>[4x]GSGSMNRTVNATTPLGDKLKFKSLKGHEQLSDLFEWTVEFVSDSPGLVLEDLLGKTISLEVETSAAPRYMHGVITAFKLVHRETQTRRYYIYEATVRPWLWYSTQVTDNRIFQDQTAVQIITQVLQAYDYPIENRLVGQYRKWGYSVQFQESDFNFISRLMEHEGIYYWFRHEKDQHVLVLMDDAHSHAPLPVMPDIPFYPDDTRSVPLEEYIRDWQIAGELTPTTYSTMDYDFQKPQAEMSARRWVKNQNTQGLDLDWYDPMGGYVDSADSDHYARVHLESMQCLQEQAWAVSNVRNLAPGYTFSLKYYPNSEENKSYLILRAEYDFRDPSYASAGGVQENATFVIRSQHIPASVQFRAPRSTPAPRMSGPQTATVVGPDGQEIWTDKYGRIKVQFHWDRQGAMDENSSCWLRVSSPWAGGGFGGVQIPRVREEVVVDFINGDVDRPIAVGRVYNASNMPPVSLPENATQSGFLTRTKNGTPENANKMLFEDSQGNELLSMVAEKDMNTHVKNNQQHDVVGNAVSSIGGLRSHTAHSTSSITMASGAVKSYQSNHNRTVQASLDDSVGGNLEQTLSDGVDETITGAHSHTVSGAASHQLLGLHVNTTTQDVETVNGTVTETVSADETTNVT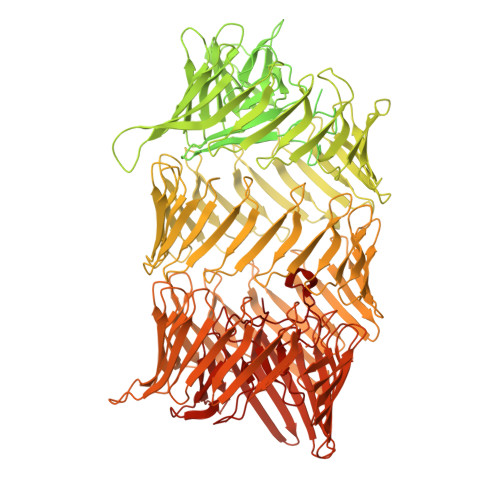SSSELEAADITLETPSLYKESTKQDININAGGSLDIQSTGPGIIQTPTDIEKESPANLEAAVMLDNNTVNREDKYILKLNLDAMSDVMVSGAKTDRNIADLAFYGMGGTMQLANVGIYGASIQMGSSDQKMGLASLSITGLELDKGFKIKTMGAGGRSGYKGKHRAAGGGRGPRGGKGGRHRAGNKGDPKKPHADCKECRGRVGGSIGLDVGDERFSHLDFVLPGVFPLEWNRTYRSNMTAKDGQGELGPRWITAFTLVVLPLETGGYEYISEVGRAVSVIELEPGQEWYDRTEELIWRRPDVDTLEVSQKYQRTETFERSGDVFRLKTIADRAGNQAQLIYDAENGFLVRVETAIQTVHLDHDAHGRITTIWHEVTGDDGTPLRRTLARYQYDEAHDLVAAVDQYERTHTYAYQNHLITRYSDKTGRGINLEWDGDHPQAKCVREYRDDGSNLLRFRWDESESKTYVTDALSATTVYTFDAHNYIIHIDFADGTRQSRIRDEFHNIVEVRYPDDSFEKYEYDEFDNILKLTRADHTTVGWEYDQYSQITKIVDPGGNIWTRDYDQFGNMIRETDPKGHTSEFQYTAEGLLIQSVNPAGGVSTLSYNPAGLLIRYSDCSNKTRRWEYDLLGRTVKQTDPCGNAESYEYNRYGFINEVRRPDGSVLTLDFDEEGRLLSFIDPIDNLTVYAYDGAGRLARKTDPLKQDFHYNYDKKGRLASLQDENGAQFTFQFDPVDRLIRTVGFDGKVKKYNYDKPTGLLFSMEDADRETHFEYDVMGQLLKRRAGHLVDSFEYDISNRIIRAHNEYCDQHFEYDVLNNPIRETHIYNAFGQNREYVWENEFDELSNRLTTRRPSGEKVSWLRYGAGHVHGILLDDQEVLSFERDNSHRAVRKRQSNSLLAVTNYDVMGRVKEQKLNLAQGNRTNLRSRQYAYGLDGSLVAIEDSRHGTTTYRYDALDRLVSATAFNETELFAFDPASNLVDRDKTERSKPANTFPKNVSKVLGNILKRCAGMHFEYDAQGNLIRKRKPDSLQEFEWDEFGRLRKTVNTDLNSKHVSEAEYIYDTFDRRIGKVNQQETSGAAVTFYGWDGHHLAFEESTVGDAVDKTHYLYEENSFVPLIQYQYSADNTIAEGRNHLSVSHYQCDHIGTPQLLTDDNGHIVWEGRYSALGKQLDSIGGDAGVAGGQNNLCYQGQYYDRESGLHYNRFRYYDPDIGRFIQQDPIGLFGDSNFYTYAPNTANWIDPFGL>GPHMEAVESGVAPPPAVRTARTDLPALASPKHSAEEPQTLLETTVMVSTKMPPHEPQVRPLGVYVRTGRGGPNGVTRVVLVRLTDPTDPFFLFELELLEDDYNAFKQHLELLVDFHGFPRYLVGMLRDIADGASAYELSFVLNSAAVGDSNRGTLRVLETTDEKTVEHISLVLLRQGDAGLKRYLAERFQHYEQSFRASEASRAVITAELQEKIGDLQAANDALRA[4x]

SAS-6 organizes the rotationally ninefold symmetric cartwheel, an early assembly intermediate of centrioles that participates in establishing their symmetry and diameter. The cartwheel is organized through the homo-oligomerization of the highly conserved centriolar protein SAS-6. High-resolution crystal structures of zebrafish and C. reinhardtii SAS-6 fragments together with biochemical and biophysical characterizations demonstrated that two dimerization interfaces in SAS-6 mediate this oligomerization: a coiled-coil domain that forms a rod-like parallel dimer; and a globular N-terminal domain that forms a curved head-to-head dimer. SAS-6 is a highly conserved protein that is found in all eukaryotes that have cilia/flagella during some of their life-cycle stages.

However, by introducing the F257E mutation to strongly weaken head-to-head dimerization we managed to crystallize construct Lm SAS-697–320 F257E that contained the N-terminal head domain and the first seven heptad-repeats of the coiled-coil domain. We subsequently solved its X-ray structure to a resolution of 2.9 Å. The asymmetric unit of the crystal contained four molecules that were highly similar to each other and superposed with an rmsd of 1.17 ± 0.50 Å in secondary structure matching with 165 ± 16 selected pairs. The crystal structure revealed that the L. major SAS-6 coiled-coil domain is a parallel dimer and packs via conserved interactions against the N-terminal head-domains as seen in other SAS-6 homologues. The F257E mutation abolishes head-to-head dimerization in solution, yet, in the crystal, due to the high protein and precipitant concentrations, some of the SAS-6 molecules present are found nevertheless in head-to-head dimers and form a curved octamer. In this octamer residues Y215 are also swung into their own hydrophobic pockets, while E257 point away from them. These data suggest that the closed Y215 conformation corresponds to a low-affinity dimerization state of the head domains and might therefore constitute a potential regulatory mechanism of SAS-6 oligomerization. The presence of curved SAS-6 octamers in the crystal of the Lm SAS-697–320 F257E mutant that is strongly impaired in its ability to form head-to-head dimers suggests that wild-type versions of SAS-6 would adopt even larger assemblies.>[2x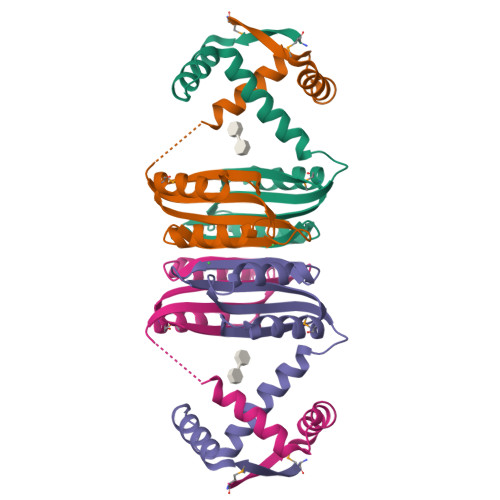]MQRVTITLDDDLLETLDSLSQRRGYNNRSEAIRDILRSALAQEATQQHGTQGFAVLSYVYEHEKRDLASRIVSTQHHHHDLSVATLHVHINHDDCLEIAVLKGDMGDVQHFADDVIAQRGVRHGHLQCLPKED>MNSSLPSLRDVFANDFRIGAAVNPVTIEMQKQLLIDHVNSITAENHMKFEHLQPEEGKFTFQEADRIVDFACSHRMAVRGHTLVWHNQTPDWVFQDGQGHFVSRDVLLERMKCHISTVVRRYKGKIYCWDVINEAVADEGDELLRPSKWRQIIGDDFMEQAFLYAYEADPDALLFYNDYNECFPEKREKIFALVKSLRDKGIPIHGIGMQAHWSLTRPSLDEIRAAIERYASLGVVLHITALDVSMFEFHDRRTD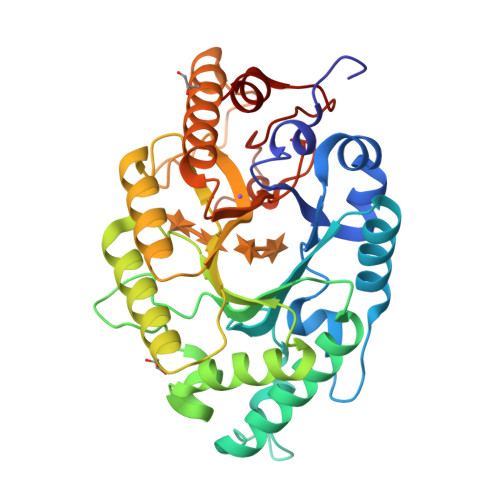LAAPTSEMIERQAERYGQIFALFKEYRDVIQSVTFWGIADDHTWLDNFPVHGRKNWPLLFDEQHKPKPAFWRAVSV[2x]> DPFTQFKQTPLPYAYDALEGAIDAKTMEIHYSKHHAGYTANLNKAIAGTPAEKESIENILAKVSQYSDAVRNNAGGHYNHELFWSILTPNKGTKPSAALQKAIDETFGSLDALKEKINAAGAARFGSGWAWLIVDN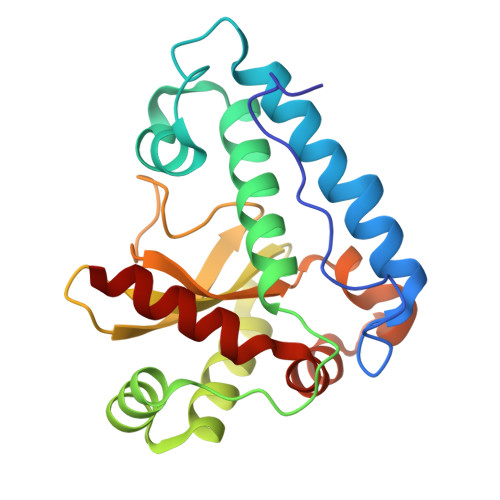GGKLQVTSTPNQDNPLMDFTKEKGTPILGIDVWEHAYYLRYQNKRADYLTTIWDVINWEEVSARYEKALK> GSHMKNSVSVDLPGSMKVLVSKSSNADGKYDLIATVDALELSGTSDKNNGSGVLEGVKADASKVKLTISDDLGQTTLEVFKSDGSTLVSKKVTSKDKSSTEEKFNEKGEVSEKIITRADGT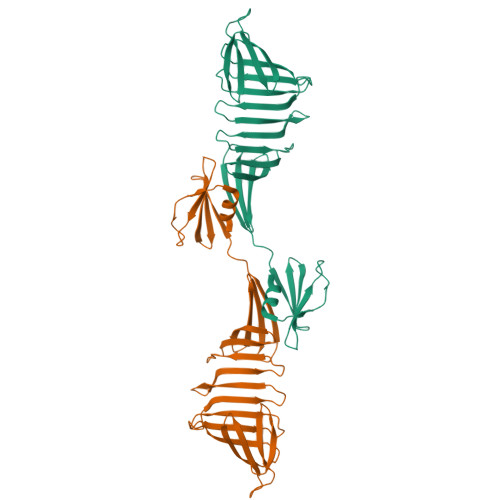RLEYTGIKSDGSGKAKEVLKGYVLEGTLTAEKTTLVVKEGTVTLSKNISKSGAVSVELNDTPPPKKTAAWNSGTSTLTITVNSKKTKDLVFTSSNTITVQQYDSNGTSLEGSAVEITKLDEIKNALK> MRKAYV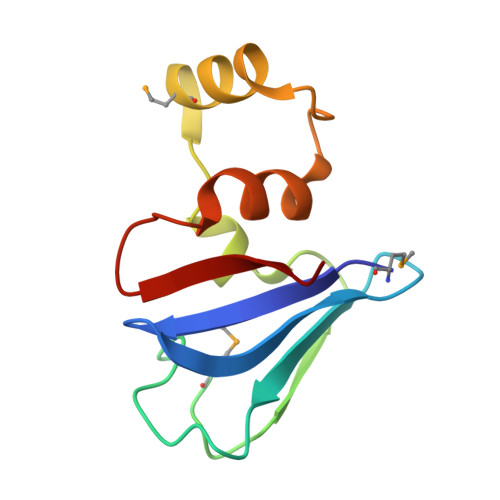SVSGIKAGILEELQGGTYQFTYFEDYHGAPVSLTMPLKNKVYDFDVFPPFFEGLLPEGIMLEALLRKYKIDKNDYFGQLILVGQDVVGAVTIEEIR>[2x]SNAMQKKSIYVAYTGGTIGMQRSDNGYIPVSGHLQRQLALMPEFH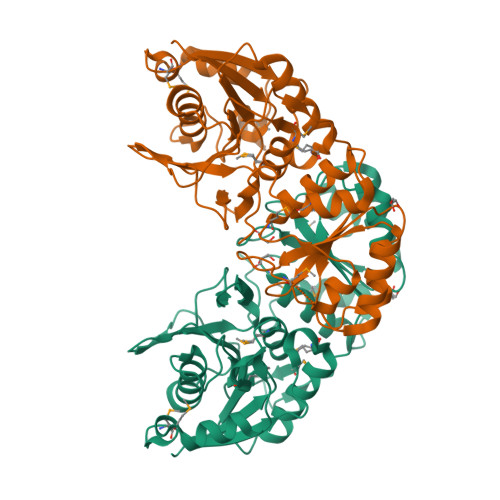RPEMPDFTIHEYAPLIDSSDMTPEDWQHIANDIQQNYDLYDGFVILHGTDTMAFTASALSFMLENLAKPVIITGSQIPLAELRSDGQTNLLNALYLAANHPVNEVSLFFNNQLFRGNRTTKAHADGFDTFASPNLSVLLEAGIHIRRQSSVVSPTSNGPLIVHRITPQPIGVVTIYPGISGAVVRNFLLQPVKALILRSYGVGNAPQKAELLDELKNASDRGIVVVNLTQCISGSVNMGGYATGNALAQAGVISGFDMTVEAALTKLHYLLSQSLSPNEIRQLMQQNLRGELTDTQ In this research, using protein-RNA crystal structures, we demonstrate that multiple structural determinants collaborate to establish the dual enzymatic activities of RlmCD, which has been previously shown to catalyze C5 methylation at both U747 and U1939 of 23S rRNA in some gram-positive bacteria. However, in S. pneumoniae and Bacillus subtilis, which both belong to gram-positive bacteria, RlmCD and its homologue YefA have been proven to be dual-functional methyltransferases to catalyze both m5U747 and m5U1939 in 23S rRNA. We previously determined the crystal structure of apo-form RlmCD, which highly resembles that of RumA and contains three individual domains, including the N-terminal TRAM domain, central domain, and C-terminal catalytic domain. In all structures, the cofactors were modeled as SAH, due to the missing electron density of the methyl group, while its density was clearly observed attaching to the base C5 atom of U747 or U1939, indicating that the complexes gained in the crystal structures all exist as the trapped enolate intermediate 3, given that E443Q eliminates the final step of proton abstraction from C5.

An 8-nt (5′-745GUUGAAAA752-3′, hereafter termed as U747L) or 12-nt (5′-743CCGUUGAAAAGG754-3′, U747SL) U747-containing RNA analogue representing the loop region of hairpin 35 alone or with two additional adjacent base pairs (743C-G754 and 744C-G753) was therefore crystalized with the construct of 1–454 of RlmCD containing a E443Q mutation, using S-adenosyl methionine (SAM) as the cofactor. The 743–754 base-pair in U747SL was modified to a G-C from an A-U to increase the stability of the RNA structure. In addition, in the RlmCD-SAH-U747SL complex structure crystalized in space group P1, each asymmetry unit contains two complex molecules that pack together through RNA-RNA intermolecular base stacking. In two complex structures of RlmCD with U747L and U747SL, the overlapped RNA loop regions show a highly similar U-shape conformation, with the U747 base flipped out of the RNA loop and engaged into the active site in the C-terminal catalytic domain of RlmCD, confirming that RlmCD recognizes U747 site majorly through the loop region of 23S rRNA hairpin 35. In addition, two extra base pairs (743C-G754 and 744C-G753) in RlmCD-SAH-U747SL show no obvious interaction with RlmCD, extending outward from the RNA catalytic groove. S2 Fig (A) In crystal of RlmCD-SAH-U747SL complex, each asymmetry unit contains two complex molecules (lime and pink) that pack together through RNA-RNA intermolecular base-stacking. (B) Superimposition of complex structures of RlmCD-SAH-U747L (marine) and RlmCD-SAH-U747SL (pink) with an RMSD for Cα atoms of 0.4 Å.

>MLKKNDIVEVEIVDLTHEGAGVAKVDGLVFFVENALPSEKILMRVLKVNKKIGFGKVEKYLVQSPHRNQDLDLAYLRSGIADLGHLSYPEQLKFKTKQVKDSLYKIAGIADVEVAETLGMEHPVKYRNKAQVPVRRVNGVLETGFFRKNSHNLMPLEDFFIQDPVIDQVVVALRDLLRRFDLKPYDEKEQSGLIRNLVVRRGHYSGQIMVVLVTTRPKVFRVDQLIEQVIKQFPEIVSVMQNINDQNTNAIFGKEWRTLYGQDYITDQMLGNDFQIAGPAFYQVNTEMAEKLYQTAIDFAELKKDDVIIDAYSGIGTIGLSVAKHVKEVYGVELIPEAVENSQKNASLNKITNAHYVCDTAENAMKKWLKEGIQPTVILVDPPRKGLTESFIKASAQTGADRIAYISCNVATMARDIKLYQELGYELKKVQPVDLFPQTHHVQTVALLSKLDVD[2x]>[2x]GM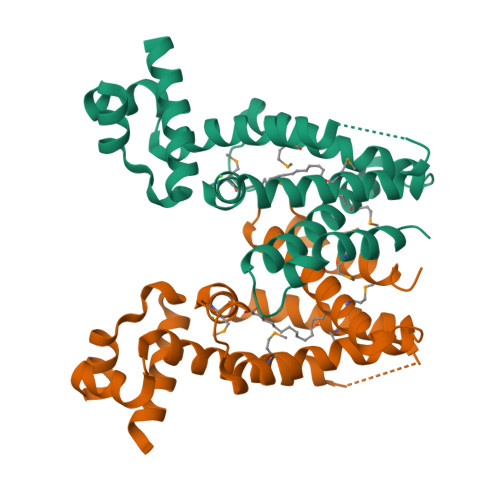AGKVEARKAALREKLIDLAEAQIEAEGLASLRARELARQADCAVGAIYTHFQDLNALTLEVNGRTFARLGAAVGAVVADGQDDHPNERLIAMSHAYLAFAREHPKLWRALFDVEMRSDGPVPQWYGHAMAQLFSYITTPLAKIFPESDDAELDLMTRTLFSSVHGIVLLGLENRISGVPGEQLKTMIRLLLEQVGR> GAMGSTIYNLEPQPTGAVIIHTTQGDLKVELFAKQTPLTCRNFLQHSLDGYYDGTIFHRLVPGFIIQGGDPTGTGHGGESIYDGGAFSGDLDPWPMDQRKGHNAGPMGVNFKDEF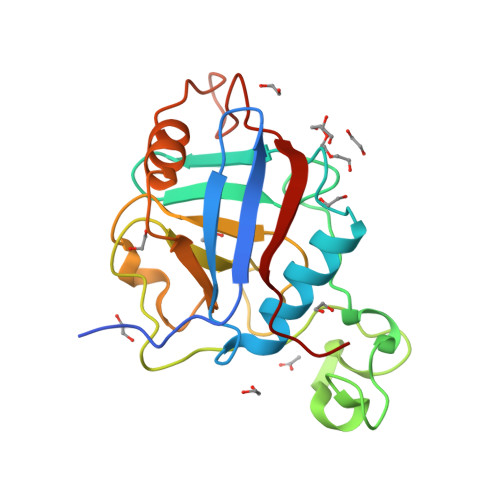HSRLKFNRRGLLGMANEGAPDTNGSQFFFTLGKAEELNNKNTLFGRVAAGDTIYNLMKWGEAELIEGTERPQYPVKITNIEILLNPFPD>MNELVDTTEMYLRTIYDLEEEGVTPLRARIAERLDQSGPTVSQTVSRMERDGLLRVAGDRHLELTEKGRALAIAVMRKHRLAERLLVDVIGLPWEEVHAEACRWEHVMSEDVERRLVKVLNNPTTSPFGNPIPGLVELGVASENLYF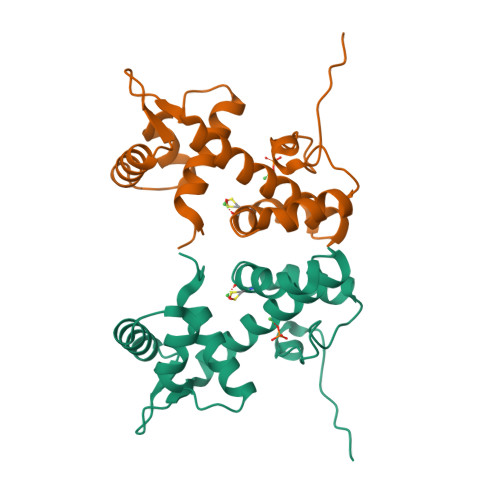QGGGHHHHHH[2x]>[2x]MIAAQLLAYYFTELKDDQVKKIDKYLYAMRLSDETLIDIMTRFRKEMKNGLSRDFNPTATVKMLPTFVRSIPDGSEKGDFIALDLGGSSFRILRVQVNHEKNQNVHMESEVYDTPENIVHGSGSQLFDHVAECLGDFMEKRKIKDKKLPVGFTFSFPCQQSKIDEAILITWTKRFKASGVEGADVVKLLNKAIKKRGDYDANIVAVVNDTVGTMMTCGYDDQHCEVGLIIGTGTNACYMEELRHIDLVEGDEGRMCINTEWGAFGDDGSLEDIRTEFDREIDRGSLNPGKQLFEKMVSGMYLGELVRLILVKMAKEGLLFEGRITPELL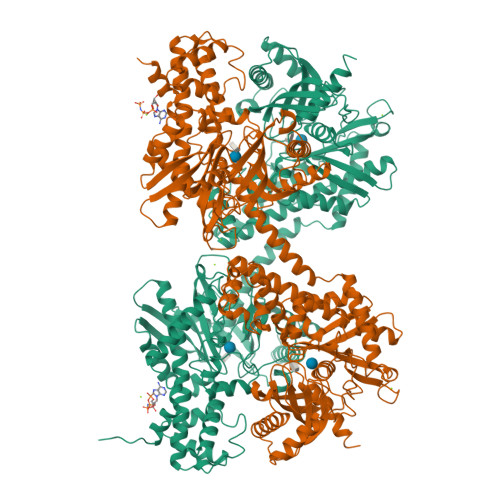TRGKFNTSDVSAIEKNKEGLHNAKEILTRLGVEPSDDDCVSVQHVCTIVSFRSANLVAATLGAILNRLRDNKGTPRLRTTVGVDGSLYKTHPQYSRRFHKTLRRLVPDSDVRFLLSESGSGKGAAMVTAVAYRLAEQHRQIEETLAHFHLTKDMLLEVKKRMRAEMELGLRKQTHNNAVVKMLPSFVRRTPDGTENGDFLALDLGGTNFRVLLVKIRSGKKRTVEMHNKIYAIPIEIMQGTGEELFDHIVSCISDFLDYMGIKGPRMPLGFTFSFPCQQTSLDAGILITWTKGFKATDCVGHDVVTLLRDAIKRREEFDLDVVAVVNDTVGTMMTCAYEEPTCEVGLIVGTGSNACYMEEMKNVEMVEGDQGQMCINMEWGAFGDNGCLDDIRTHYDRLVNEYSLNAGKQRYEKMISGMYLGEIVRNILIDFTKKGFLFRGQISETLKTRGIFETKFLSQIESDRLALLQVRAILQQLGLNSTCDDSILVKTVCGVVSRRAAQLCGAGMAAVVDKIRENRGLDRLNVTVGVDGTLYKLHPHFSRIMHQTVKELSPKCNVSFLLSEDGSGKGAALITAVGVRLRTEASS> SNAGVALPSPQNGEQPNPTGPALNVDVPPRDAAERVT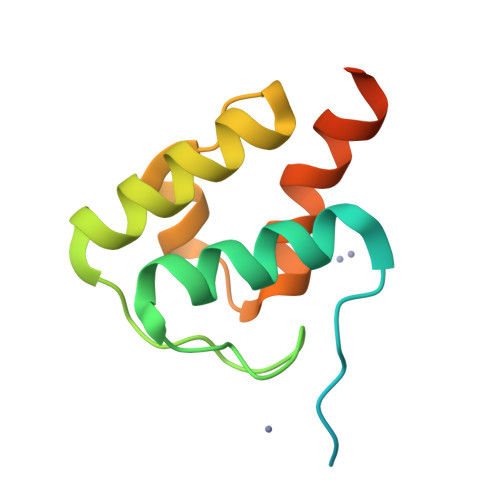FATWAIVTGKSPGGIFNELPRLDDEAAAKIAQRLSERAEGPITAEDVLTSSNIEALADKVRTYLEAGQIDGFVRTLRA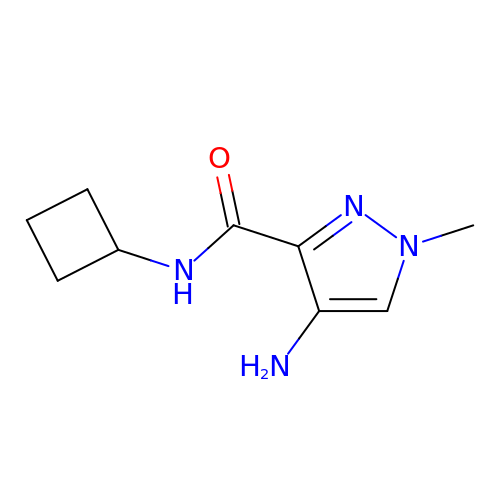4-amino-N-cyclobutyl-1-methyl-1H-pyrazole-3-carboxamide | C9 H14 N4 O | NILOPFIVQCAHIP-UHFFFAOYSA-N>MMITLDHVTKQYKSSARPALDDINVKIDKGEFVFLIGPSGSGKSTFMRLLLAAETPTSGDVRVSKFHVNKLRGRHVPKLRQVIGCVFQDFRLLQQKTVYDNVAFALEVIGKRTDAINRVVPEVLETVGLSGKANRLPDELSGGEQQRVAIARAFVNRPLVLLADEPTGNLDPETSRDIMDLLERINRTGTTVLMATHDHHIVDSMRQRVVELSLGRLVRDEQRGVYGMDR[2x];>MRFGFLLNEVLTGFRRNVTMTIAMILTTAISVGLFGGGMLVVRLADSSRAIYLDRVESQVFLTEDVSANDSSCDTTACKALREKIETRSDVKAVRFLNRQQAYDDAIRKFPQFKDVAGKDSFPASFIVKLENPEQHKDFDTAMKGQPGVLDVLNQKELIDRLFAVLDGLSNAAFAVALVQAIGAILLIANMVQVAAYTRRTEIGIMRLVGASRWYTQLPFLVEAMLAATMGVGIAVAGLMVVRALFLENALNQFYQANLIAKVDYADILFITPWLLLLGVAMSGLTAYLTLRLYVRR[2x];> MRLDQRWLIARVIMRSAIGFFASFTVSSGVLAANVLADPADDALAKLNELSRQAEQTTEALHSAQLDLNEKLAAQRAADQKLADNRTALDAARARLATFQTAVNKVAAATYMGGRTHGMDAILTAESPQLLIDRLSVQRVMAHQMSTQMARFKAAGEQAVKAEQAAAKSAADARSAAEQAAAVRANLQHKQSQLQVQIAVVKSQYVALTPEERTALADPGPVPAVAAIAPGAPPAALPPGAPPGDGPAPGVAPPPGGMPGLPFVQPDGAGGDRTAVVQAALTQVGAPYAWGGAAPGGFDCSGLVMW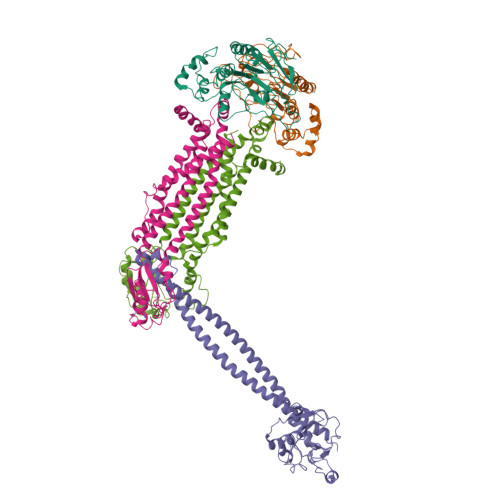AFQQAGIALPHSSQALAHGGQPVALSDLQPGDVLTFYSDASHAGIYIGDGLMVHSSTYGVPVRVVPMDSSGPIYDARRY> GALEHEKLVNYIALGEFSRETAEIALKKMPPLDTLTVHYDLQLYKINYKTQSPDGNLTIASGLVAMPIHPVGQVGIISYQHGTRFERNDVPSRNNEKNYIYLAAYGNSAGYMTVMPDYLGLGDNELTLHPYVQAETLASSSIDMLFAAKE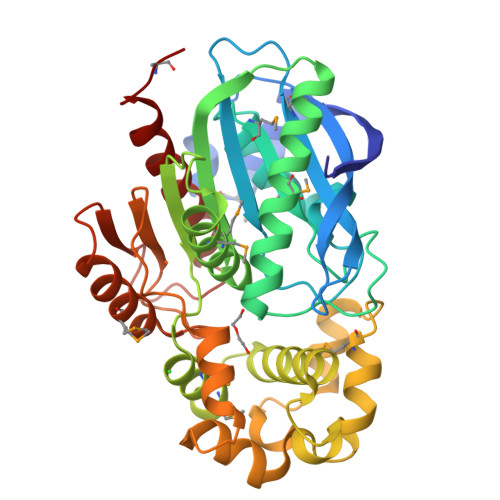LANRLHYPISDKLYLAGYSEGGFSTIVMFEMLAKEYPDLPVSAVAPGSAPYGWEETMHFVMLEPGPRATAYLAYFFYSLQTYKSYWSGFDEIFAPPYNTLIPELMDGYHAVDEILQALPQDPLLIFQPKFSNGIISKTDRNTEILKINFNHYDFKPTAPLLLVGTKGDRDVPYAGAEMAYHSFRKYSDFVWIKSVSDALDHVQAHPFVLKEQVDFFKQFERQEAMNK> MGSSHHHHHHSQDPDVEDLFSSLKHIQHTLVDSQSQEDISLLLQLVQNRDFQNA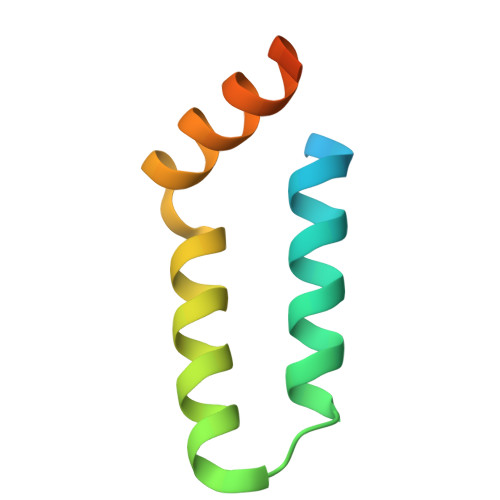FKIHNAVTVHMSKASPPF> SLSDFSVASRDVNHNNICAGLSTEWLVMSSDGDAESRMDHLDYNGEGQSRGSERHQVYNDALRAALSNDDEAPFFTASTAVIEDAGFSLRREPKTVHASGGSAQLGQTVAHDVAQSGRKHLLSLRFANVQGHAIACSCEGSQFKLFDPNLGEFQSSRSAAPQLIKGLIDHYNS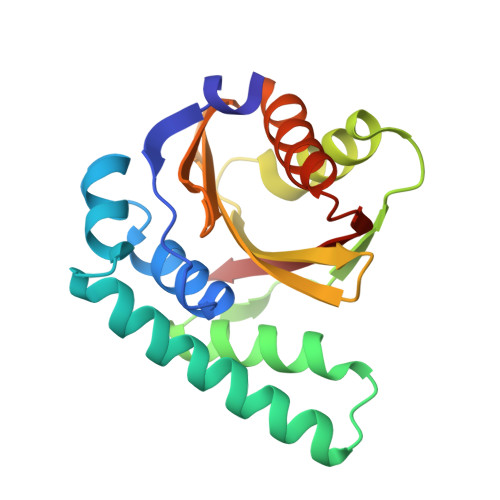LNYDVACVNEFRVSV> VVGGMSAEPGAWPWMVSLQIFMYH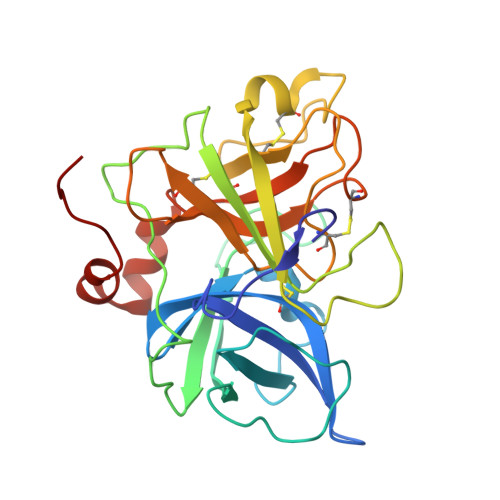NNRRYHTCGGILLNSHWVLTAAHCFKNKKKVTDWRLIFGANEVVWGSNKPVKPPLQERFVEEIIIHEKYVSGLEINDIALIKITPPVPCGPFIGPGCLPQFKAGPPRAPQTCWVTGWGYLKEKGPRTSPTLQEARVALIDLELCNSTRWYNGRIRSTNVCAGYPRGKIDTCQGDSGGPLMCRDRAENTFVVVGITSWGVGCARAKRPGVYTSTWPYLNWIASKIGSNALQMVQLGTPPR>[2x]GPHMSTSSANEDMPVEKILEAELAVEPKTETYVEANMGLNPSSPNDPVTNICQAADKQLFTLVEWAKRIPHFSELPLDDQVILLRAGWNELLAASASHRSIAVKDGILLTTGLHVHRNSAHSAGVGAIFDRVLTELVSKMRDMQMDKTELGCLRAIVLFNPDSKGLSNP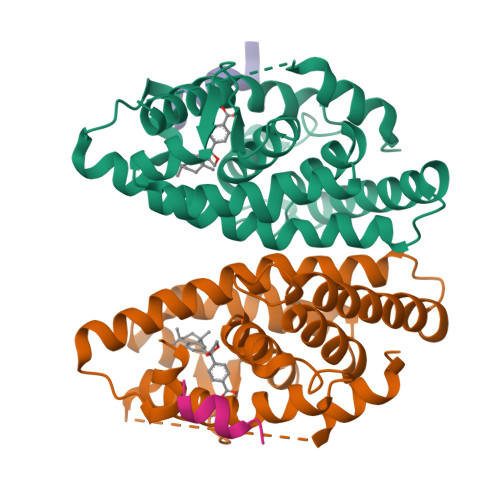AEVEALREKVYASLEAYCKHKYPEQPGRFAKLLLRLPALRSIGLKCLEHLFFFKLIGDTPIDTFLMEMLEAPHQAT;>KHKILHRLLQDSS[2x]>SARILVVDDIEANVRLLEAKLTAEYYEVSTAMDGPTALAMAARDLPDIILLDVMMPGMDGFTVCRKLKDDPTTRHIPVVLITALDGRGDRIQGLESGASDFLTKPIDDVMLFARVRSLTRFKLVIDELRQREASGRRMGVIAGAAARLDGLGGRVLIVDDNERQAQRVAAELGVEHRPVIESDPEKAKISAGGPVDLVIVNAAAKNFDGLRFTAALRSEERTRQLPVLAMVDPDDRGRMVKALEIGVNDILSRPIDPQELSARVKTQIQRKRYTD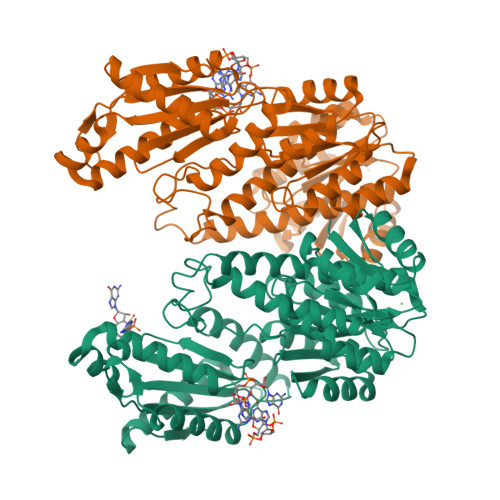YLRNNLDHSLELAVTDQLTGLHNRRYMTGQLDSLVKRATLGGDPVSALLIDIDFFKKINDTFGHDIGDEVLREFALRLASNVRAIDLPCRYGGEEFVVIMPDTALADALRIAERIRMHVSGSPFTVAHGREMLNVTISIGVSATAGEGDTPEALLKRADEGVYQAKASGRNAVVGKAAHHHHHH[2x]> SMHLICQSGDVLSARYEIVDTLGEGAFGKVVECIDHKAGGRHVAVKIVKNVDRYCEAARSE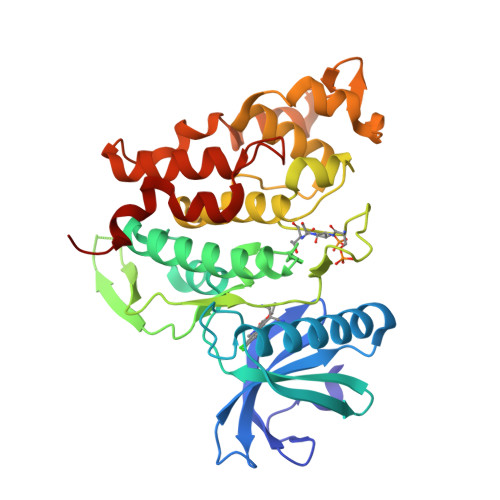IQVLEHLNTTDPNSTFRCVQMLEWFEHHGHICIVFELLGLSTYDFIKENGFLPFRLDHIRKMAYQICKSVNFLHSNKLTHTDLKPENILFVQSDYTEAYNPKIKRDERTLINPDIKVVDFGSATYDDEHHSTLVSTRHYRAPEVILALGWSQPCDVWSIGCILIEYYLGFTVFPTHDSKEHLAMMERILGPLPKHMIQKTRKRKYFHHDRLDWDEHSSAGRYVSRACKPLKEFMLSQDVEHERLFDLIQKMLEYDPAKRITLREALKHPFFDLLKKSI By integrating comparative genomics, transcriptomics, functional genetics, and metabolomics analysis, we identified a unique polyyne resistance gene, masL (encoding acetyl-CoA acetyltransferase), in the biosynthesis gene cluster of antifungal polyynes (massilin A 1, massilin B 2, collimonin C 3, and collimonin D 4) of Massilia sp. YMA4. Crystallographic analysis indicated that bacterial polyynes serve as covalent inhibitors of acetyl-CoA acetyltransferase. The monomer of MasL shares the general fold architecture reported in the type II biosynthetic thiolase family. MasL consists of three domains: an N-terminal α/β domain (N-domain, residues 1–121 and 251–271), a loop domain (L-domain, residues 122–250), and a C-terminal α/β domain (C-domain, residues 272–394).

To investigate how bacterial polyynes target acetyl-CoA acetyltransferase, we solved the crystal structures of MasL in its apo and two holo (bound collimonin C 1 and collimonin D 2) forms at 1.78 Å, 1.66 Å, and 1.40 Å resolution, respectively. The asymmetric unit (space group P1 for apo MasL and MasL-collimonin D complex; P21 for MasL-collimonin C complex) of both structures contains a tetramer of the protein, as observed in solution. In the MasL-collimonin C complex, the conjugated polyyne tail extended into the MasL substrate binding site and formed a covalent bond between the terminal carbon (C16) of the alkyne moiety and the reactive cysteine sulfhydryl moiety of Cys90 via nucleophilic addition. Thus, the terminal alkyne was essential for polyyne activity through covalent modification on the reactive cysteine sulfhydryl group of acetyl-CoA acetyltransferases. In the further comparative analysis of the polar interactions in the activation pocket of MasL in MasL-collimonin C and MasL-collimonin D complex, the C(7)OH moiety of collimonin C/D 1, 2, His158 of MasL, and a water molecule formed a strong polar interaction network, including a direct hydrogen bond (3.00–3.16 Å) and a water-mediated hydrogen bond between C(7)OH and His158. Furthermore, although there was no significant induced-fit within the pocket, the collimonin C/D 1, 2 caused the Arg135 on the tetramerization loop to swap and form a hydrogen bond interaction and salt bridge, respectively, across the two subunits within the binding site. The C6 chiral center of collimonin C/D 1, 2 is critical to forming different polar interactions. The C(6)OH of collimonin C 1 had more flexibility concerning the spatial direction (with a dihedral angle to C(7)OH from 109˚ to 170˚) and built a sophisticated polar interaction network with the amide of Pro249 in the pantetheine loop, Arg135, and multiple water molecules. The polar interaction network derived from C(6)OH of collimonin C 1 further affected the distal carboxyl group binding model.

>MVKDEIVISSALRTPIGAFSGTLKDTPAAALGAHVVKTLLERTGLAPERVDEVVMGNVLQAGNGMNVARQVAVNGGLPVAVPAHTVNRVCGSGAQAVVTAYAQIRSGLSNLVIAGGVENMDQAPYLMPSLRHGARMGHTQALDALLRDGLNDAFSDQHSGWHTEDLVAKYEVSREAQDRFAATSQQRFAAAQAAGWFEGEIVPVTITTRKGETVFAKDEANRPDTTEAGLAKLRPAFRKDGTITAGNAPGLNAGAAAMIVSSHATATELGLQPQLVIRGIGVAAVEPGLFGFGPVPAIKLALAQAQWQVQDVDRFEVNEAFAAVGLVVRDELGIAPERFNVDGGAIAHGHPIGATGAILLTKVAHALRRTSERRAVVSLCIGGGQGIALALERVKLAAALEHHHHHH[4x]> MADIYPLGKTHTEELNEIIVESAKEIAEPDTTMIQKLIDEHNPEPLLKGVRYYMCENDIEKKRRTYYDAAGQQLVDDTKTNNRTSHAWHKLFVDQKTQYLVGEPVTFTSDNKTLLEYVNELADDDFDDILNETVKNMSNKGIEYWHPFVDEEGEFDYVIFPAEEMIVVYKDNT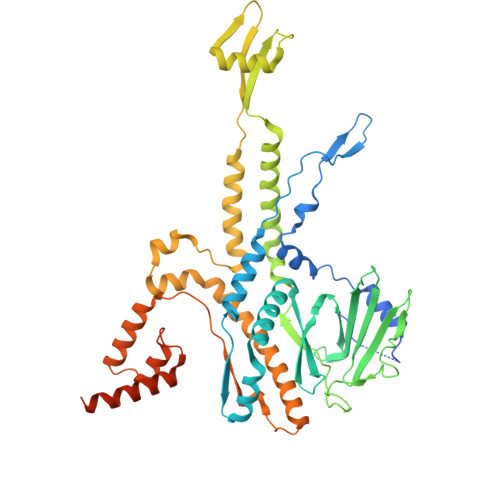RRDILFALRYYSYKGIMGEETQKAELYTDTHVYYYEKIDGVYQMDYSYGENNPRPHMTKGGQAIGWGRVPIIPFKNNEEMVSDLKFYKDLIDNYDSITSSTMDSFSDFQQIVYVLKNYDGENPKEFTANLRYHSVIKVSGDGGVDTLRAEIPVDSAAKELERIQDELYKSAQAVDNSPETIGGGATGPALENLYALLDLKANMAERKIRAGLRLFFWFFAEYLRNTGKGDFNPDKELTMTFTRTRIQNDSEIVQSLVQGVTGGIMSKETAVARNPFVQDPEEELARIEEEMNQYAEMQGNLLDDEGGDDDLEEDDPNAGAAESGGAGQVS> MTLIYKILSRAEWDAAKAQGRFEGSAVDLADGFIHLSAGEQAQETAAKWFRGQANLVLLAVEAEPLGEDLKWEASRGGARFPHLYRPLLVSE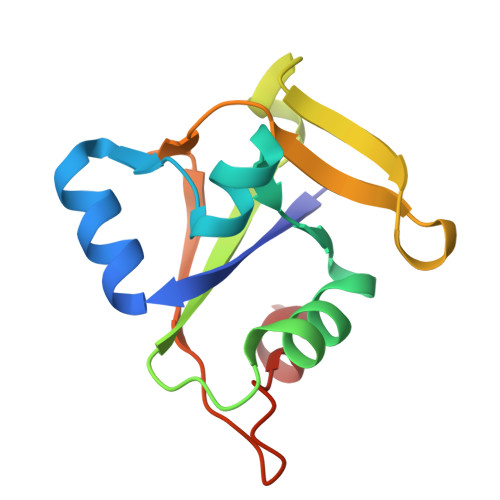VTREADLDLDADGVPQLGDHLAL> MERNHWNEKSSGAKRSRERDLTLSTIRSILAADERLRIKASSYLGVGRGVDDEAVIDIFPTGQTMSFLRLLHGFLGTCRGQSMHQVLRDPCVLRKQLLYGVCKTLFDTITVRRVAEEWKLHAALFPYRALDEEDLEQYLLVWSASLRQSVQTGVLGALRDILYQYADNDDYGLYVDWCVTVGLVPLLDVKTKPSEAAERAQFVRAAVQRATETHPLAQDLLQANLALLLQVAERLGAVRVANAPEVRVFKKVRSERLEAQLRGKHIRLYVAAEPLAYERDKLLFTTPVAHLHEEILRYDGLCRHQKICQLLNTFPVKVVTASRHELNCKKLVEMMEQHDRGSDAKKSIMKFLLNVSDSKSRIGIEDSVESFLQDLTPSLVDQNRLLPARGPGGPGVVGPGGAVVGGPAGHVGLLPPPPGPAAPERDIRDLFKKQVIKCLEEQIQSQVDEIQDLRTLNQTWENRVRELRDLLTRYASRREDSMSLGARDAELYHLPVLEAVRKARDAAPFRPLAVEDNRLVANSFFSQFVPGTESL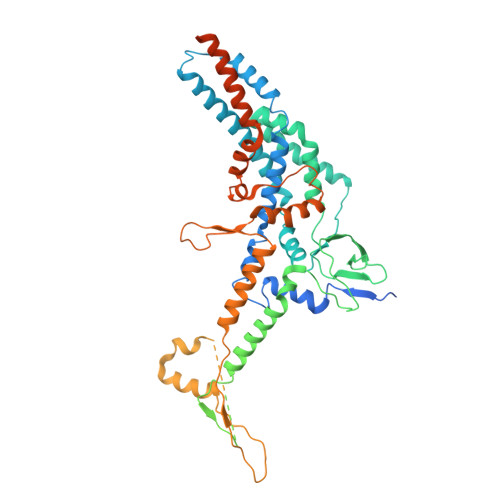ERFLTQLWENEYFRTFRLRRLVTHQGAEEAIVYSNYTVERVTLPYLCHILALGTLDPVPEAYLQLSFGEIVAAAYDDSKFCRYVELICSREKARRRQMSREAAGGVPERGTASSGGPGTLERSAPRRLITADEERRGPERVGRFRNGGPDDPRRAGGPYGFH> MASVHGTTYELLRRQGIDTVFGNPGTNELPFLKDFPEDFRYILALQEACVVGIADGYAQASRKPAFINLHSAAGTGNAMGALSNAWNSHSPLIVTAGQQTRAMIGVEALLTNVDAANLPRPLVKWSYEPASAAEVPHAMSRAIHMASMAPQGPVYLSVPYDDWDKDADPQSHHLFDRHVSSSVRLNDQDLDILVKALNSASNPAIVLGPDVDAANANADCVMLAERLKAPVWVAPSAPRCPFPTRH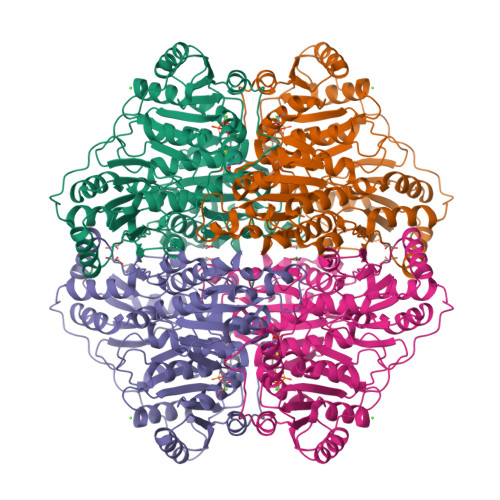PCFRGLMPAGIAAISQLLEGHDVVLVIGAPVFRYHQYDPGQYLKPGTRLISVTCDPLEAARAPMGDAIVADIGAMASALANLVEESSRQLPTAAPEPAKVDQDAGRLHPETVFDTLNDMAPENAIYLNESTSTTAQMWQRLNMRNPGSYYFCAAGGLGFALPAAIGVQLAEPERQVIAVIGDGSANYSISALWTAAQYNIPTIFVIMNNGTYGALRWFAGVLEAENVPGLDVPGIDFRALAKGYGVQALKADNLEQLKGSLQEALSAKGPVLIEVSTVSPVKRSHHHHHH>MKKITLLLAGSALLLSGCAGVKSSFDCDATTSDTCMTMTKANQLARDKAAKQAGKPAAGGLPSLVNLPATSAVEVPSASRSAVTPPSGTRTVSTTPPVSAGTSAGVNTNTTTSTLTPRPVAGTPVTTTPSSVAYRPVVSVVTPTPSCQNVRCDNPGTVHPQRSRDQIATVWIAPWVDSDNAFHQPGRVSFVVSPADWVLPARVN[26x];>[13x]PGMMDSQEFS;>[26x]AQSPATISLPQGGQFRLSISNTDPNMIFIPGDKVTAITAPGGM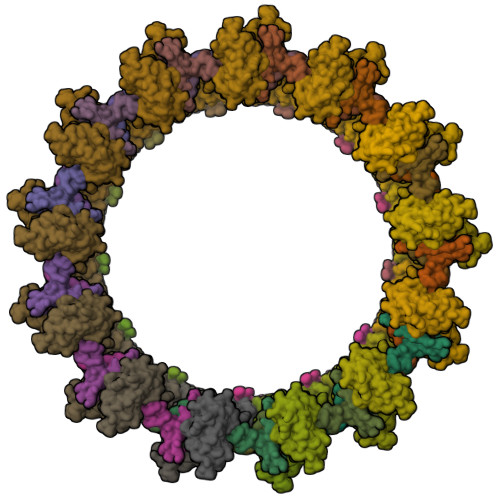LADKRLTTAGGVLFTSVATRTFTIFVETALGQTFSVVATPVKGEGRVYRLMSAEPPSRPETRKWETAQAYEKLLISLNRAVLTGDIPDGYGEVKPLSDGIRLPGGFSVTPLKAWAGDQLRADRYELRNANTWGVALREQDFWKPGVRAVMFDNNAQTLMGGGRMTVTVIRGNG> KTSDANETEDHLESLICKVGEKSACSLESNLEGLAGVLEADLPN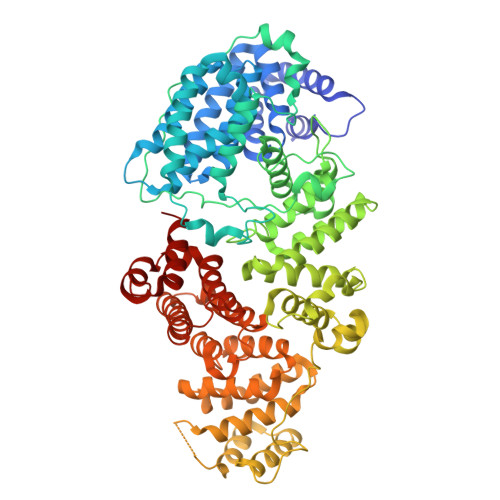YKSKILRLLCTVARLLPEKLTIYTTLVGLLNARNYNFGGEFVEAMIRQLKESLKANNYNEAVYLVRFLSDLVNCHVIAAPSMVAMFENFVSVTQEEDVPQVRRDWYVYAFLSSLPWVGKELYEKKDAEMDRIFANTESYLKRRQKTHVPMLQVWTADKPHPQEEYLDCLWAQIQKLKKDRWQERHILRPYLAFDSILCEALQHNLPPFTPPPHTEDSVYPMPRVIFRMFDYTDDPEGPVMPGSHSVERFVIEENLHCIIKSHWKERKTCAAQLVSYPGKNKIPLNYHIVEVIFAELFQLPAPPHIDVMYTTLLIELCKLQPGSLPQVLAQATEMLYMRLDTMNTTCVDRFINWFSHHLSNFQFRWSWEDWSDCLSQDPESPKPKFVREVLEKCMRLSYHQRILDIVPPTFSALCPSNPTCIYKYGDESSNSLPGHSVALCLAVAFKSKATNDEIFSILKDVPNPNQDDDDDEGFSFNPLKIEVFVQTLLHLAAKSFSHSFSALAKFHEVFKTLAESDEGKLHVLRVMFEVWRNHPQMIAVLVDKMIRTQIVDCAAVANWIFSSELSRDFTRLFVWEILHSTIRKMNKHVGAQSEQKNLFLVIFQRFIMILTEHLVRCETDGTSVLTPWYKNCIERLQQIFLQHHQIIQQYMVTLENLLFTAELDPHILAVFQQFCALQA>[2x]HHHHHHHHENLYFQGDPTQFEERHLKFLQQLGKGNFGSVEMCRYDPLQDNTGEVVAVKKLQHSTEEHLRDFEREIEILKSLQHDNIVKYKGVCYSAGRRNLKLIMEYLPYGSLRDYLQKHKERIDHIKL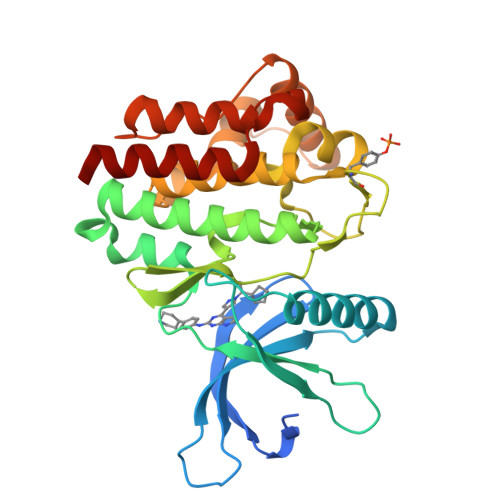LQYTSQICKGMEYLGTKRYIHRDLATRNILVENENRVKIGDFGLTKVLPQDKEYYKVKEPGESPIFWYAPESLTESKFSVASDVWSFGVVLYELFTYIEKSKSPPAEFMRMIGNDKQGQMIVFHLIELLKNNGRLPRPDGCPDEIYMIMTECWNNNVNQRPSFRDLALRVDQIRDNMAG>MKKIEHKMVAVNGLNMHLAELGEGPTILFIHGFPELWYSWRHQMVYLAERGYRAVAPDLRGYGDTTGAPLNDPSKFSILHLVGDVVALLEAIALNEEKVFVVAHDLGAYIAWHLCLF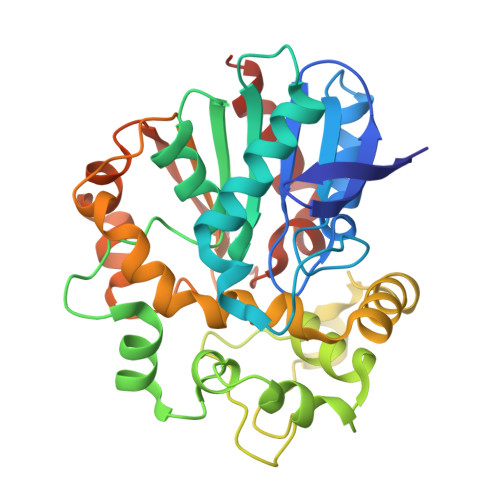RPDKVKALVNLSVHFSKRNPKMNKVEGLKAIYGEDHYVSRFQVPGEIEAEFAPIGAKSVLKKILTYRDPAPLYFPKGKGLEAIPDAPVALSSWLSEEELDYYANKFEQTGFTGAVNYYRALPINWELTAPWTGAQVKVPTKFIVGEFDLVYHIPGAKEYIHNGGFKKDVPLLEEVVVLEGAAHFVSQERPHEISKHIYDFIQKFTSHHHHH[2x]> MGMSPKKNSASRPSNNGGGGKTGGGNGNVSHRTDNEQSGNNLSERIIANESLLATESERHATSKSLYGDCTARISGNLSCIHDRVRLRAYESVLRSIKGKSVLHLGCGMGLVSMIAARSLASAVVAVDRSAIVDAAQVVANKNGLNNISFFRGALVDVVQNFPVRQFDVIICEWMGPFLINDPLLEEALYARNNLLASNGVMCPDSSSIHV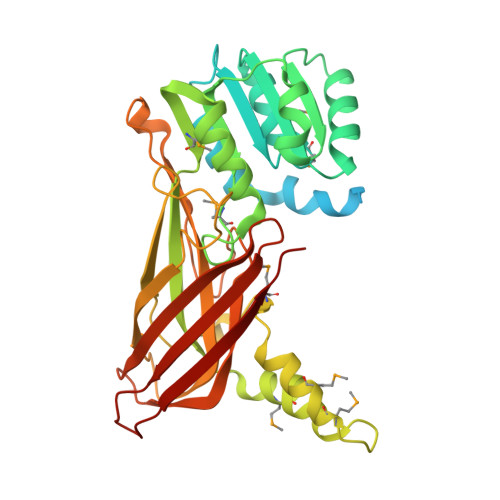VGVSDYCFHMDTVEFWGNVYGFKMEPMKALVQREVEMCRVPTSSIVTTTCLAHTVNIASINNLDDKSSLNDFVVPFSVRATKDTTVNFLTFYIDARFTNPHDPGANFVLGVRPGGTNPWTETSVALHEPLPLKGGEVLSGELKVCLLNPTRGITTVEVTARTSGNVVNIETKGTYNYQRY> VPTLQRDVAIVGAGPSGLAAATALRKAGLSVAVIEARDRVGGRTWTDTIDGAVLEIGGQWVSPDQTALISLLDELGLKTFERYREGESVYISSAGERTRYTGDSFPTNETTKKEMDRLIDEMDDLAAQIGAEEPWAHPLARDLDTVSFKQWLINQSDDAEARDNIGLFIAGGMLTKPAHSFSALQAVLMAASAGSFSHLVDEDFILDKRVIGGMQQVSIRMAEALGDDVFLNAPVRTVKWNESGATVLADGDIRVEASRVILAVPPNLYSRISYDPPLPRRQHQMHQHQSLGLVIKVHAVYETPFWREDGLSGTGFGASEVVQEVYDNTNHEDDRGTLVAFVSDEKADAMFELSAEERKATILASLARYLGPKAEEPVVYYESDWGSEEWTRGCYAASFDLG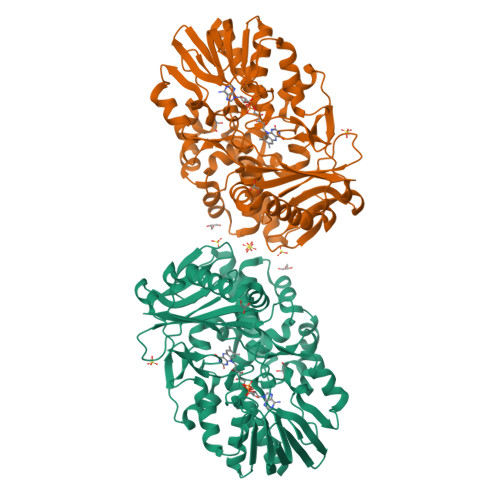GLHRYGADSRTPVGPIHFSCSDIAAEGYQHVDGAVRMGQRTAADIIARSKA>GSPEFRGVIIKQGCLLKQGHRRKNWKVRKFILREDPAYLHYYDPAGAEDPLGAIHLRGCVVTSVESNSNGRKSEEENLFEIITADEV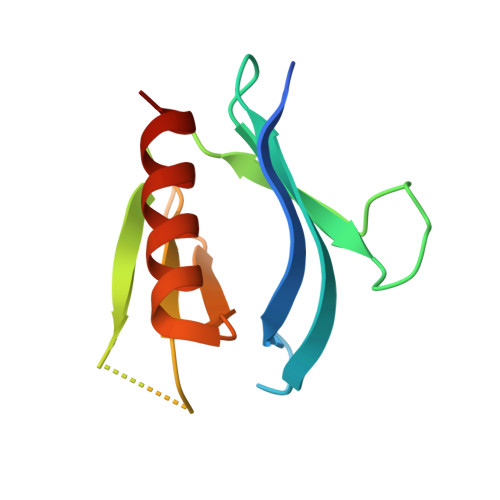HYFLQAATPKERTEWIKAIQMASRTGK[2x]>[5x]MDAFKRNLEKLAELAIRVGLNLEKGQEVIATAPIEAVD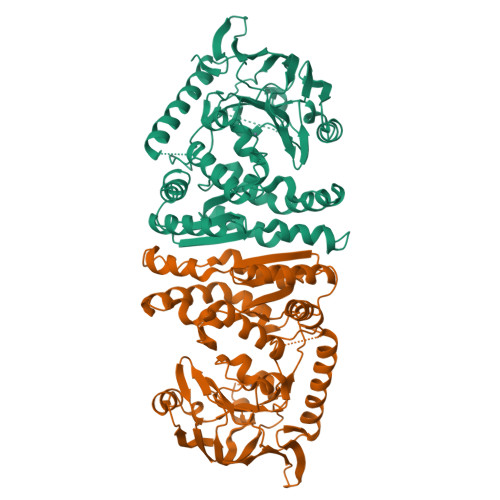FVRLLAEKAYREGASLFTVIYGDQELARKRLALAPEEGLDKAPAWLYEGMARAFREGAARLAVSGSDPKALEGLPPEKVGRAQKANARAYKPALEAITEFVTNWTIVPFAHPGWARAVFPGLPEEEAVRRLWEAIFQATRADQEDPIAAWEAHNRALHEKVAYLNARRFHALHFKGPGTDLVVGLAEGHLWQGGATATKGGRLCNPNLPTEEVFTAPHRERVEGVVRASRPLALGGTLVEGIFARFERGFAVEVRAEKGEEVLRRLLDTDEGARRLGEVALVPADNPIAKTGLVFFDTLFDENAASHIAFGQAYQENLEGRPSGEAFRKRGGNESLVHVDWMIGSEEMDVDGLYEDGTRTPLMRRGRWVV> GSHMEQLKHCN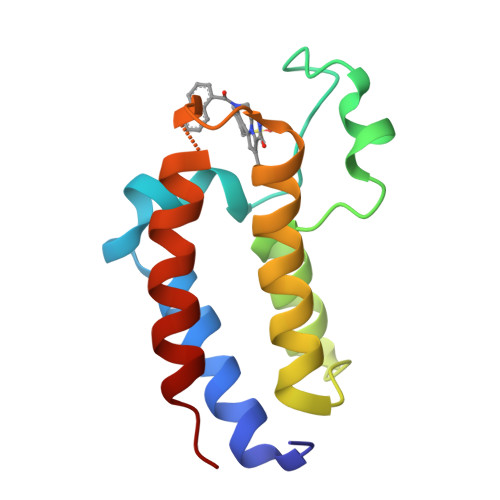GILKELLSKKHAAYAWPFYKPVDASALGLHDYHDIIKHPMDLSTVKRKMENRDYRDAQEFAADVRLMFSNCYKYNPPDHDVVAMARKLQDVFEFRYAKMPD> CELDRDPEGKDFQQPYTSFVQTKQNRDGLYALLRNTENPRMHFYQELQSDMYCTTITDGNSLAPFVNWDLGILNDHGRADEDEVSGIAGYYFVYNRLNQQANAFVNNTEAALQNQVYKNSTEIANAKSFLAEGKVLQALAIWRLMDRFSFHESVTEVNSGAKDLGVILLKEYNPGYIGPRATKAQCYDYILSRLS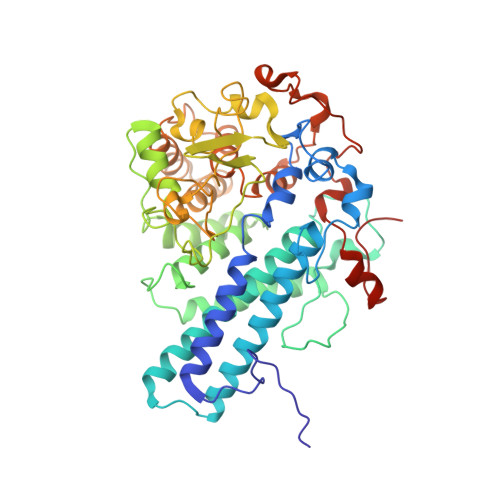EAIEVLPENRESVLYVSRDYAYALRARIYLALGEYGKAAADAKMVVDKYPLIGAADASEFENIYRSDANNPEIIFRGFASATLGSFTATTLNGAAPAGKDIKYNPSAVPFQWVVDLYENEDFRKSVYIAKVVKKDKGYLVNKFLEDKAYRDVQDKPNLKVGARYFSVAEVYLILVESALQTGDTPTAEKYLKALSKARGAEVSVVNMEALQAERTRELIGEGSRLRDMVRWSIPNNHDAFETQPGLEGFANTTPLKAQAPVGFYAYTWEFPQRDRQTNPQLIKNWPIHHHHHH> GAGCAGCCTGTUTGGACATCA;> CCAUACAU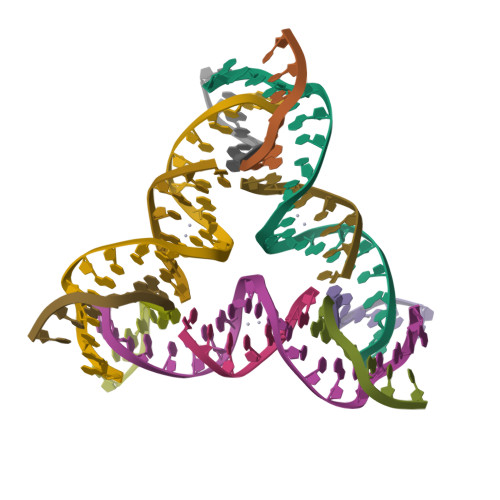ACA;> GGCTGCT;> CTGATGT2-[[7-[2,6-dimethyl-4-(3-methylphenyl)carbonyl-phenoxy]-1-methoxy-4-oxidanyl-isoquinolin-3-yl]carbonylamino]ethanoic 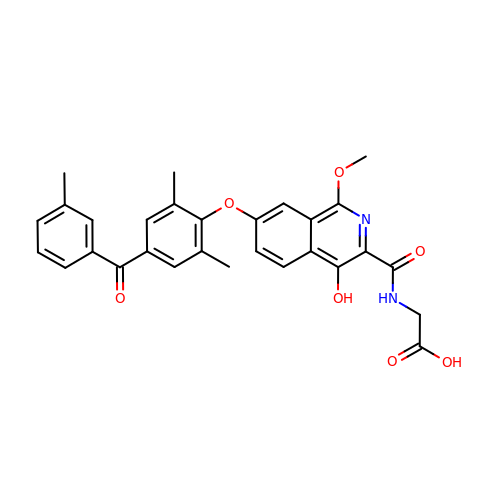acid | C29 H26 N2 O7 | MXIPXHVKKFYVCB-UHFFFAOYSA-N> MPINRPNLNLNIPPLNIVAAYDGAEIPSTNKHLKNNFNSLHNQMRKMPVSHFKEALDVPDYSGMRQSGFFAMSQGFQLNNHGYDVFIHARRESPQSQGKFAGDKFHISVLRDMVPQAFQALSGLLFSEDSPVDKWAVTDMEKVVQQARVSLGA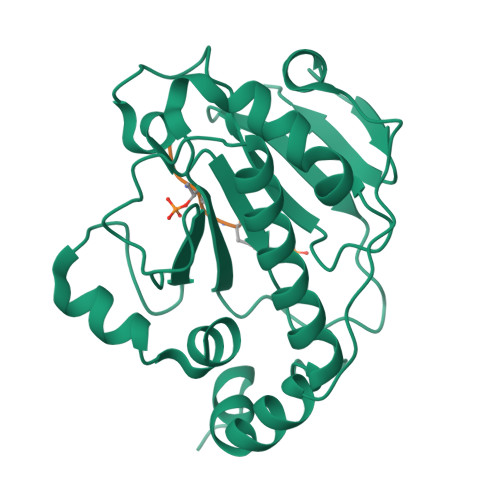QFTLYIKPDQENSQYSASFLHKTRQFIECLESRLSENGVISGQCPESDVHPENWKYLSYRNELRSGRDGGEMQRQALREEPFYRLMTE;> GEATVYA>[4x]MKADAVKI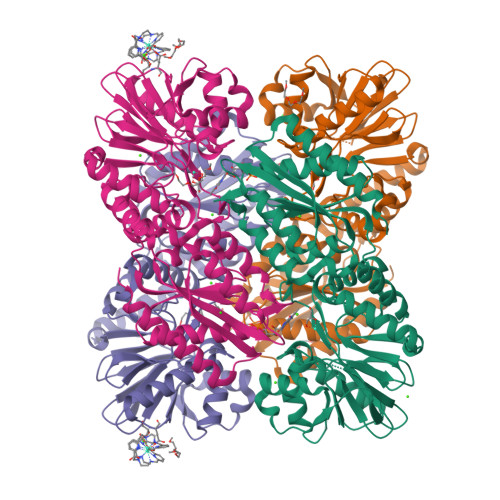ADGVYWVGVLDWDIRMYHGYTLNGTTYNAYLVFGDDKVALIDNTYPGTSAQMWGRIKDACEKEGREFKIDVIVQNHVEKDHSGALPEIHKKFPEAPIYCTEVAVEGLVKHFPSLKGAPFKVVKSLESIDLGGKTLTFLEAPLLHWPDSMFTLYAEEGILFSNDAFGQHLCFTQRFDHEIPENILMDANQKFYANLITPLSKLVLKKFKEVIELGLLEKIKMIAPSHGQIWTDPMKVIGAYQDFATGKCKDKVTIVYDTMHGSTQKMAHAFAEGIMSEGVDVKMYFLHNDERSEIVKDILDSKAFLLGAPTIYDEPFPSVGDLIYYLKGLKFNRTGLKRLALAFGSMGGNGGGTKVLAEKLKECGFEVLDEYELYYVPTEDELEKCYNMGKRLAVKVKEMKTE> MAASGLDHLKNGYRRRFCRPSRARDINTEQGQNVLEILQDCFEEKSLANDFSTNSTKSVPNSTRKIKDTCIQSPSKECQKSHPKSVPVSSKKKEASLQFVVEPSEATNRSVQAHEVHQKILATDVSSKNTPDSKKISSRNINDHHSEADEEFYLSVGSPSVLLDAKTSVSQNVIPSSAQKRETYTFENSVNMLPSSTEVSVKTKKRLNFDDKVMLKKIEIDNKVSDEEDKTSEGQERKPSGSSQNRIRDSEYEIQRQAKKSFSTLFLETVKRKSESSPIVRHAATAPPHSCPPDDTKLIEDEFIIDESDQSFASRSWITIPRKAGSLKQRTISPAESTALLQGRKSREKHHNILPKTLANDKHSHKPHPVETSQPSDKTVLDTSYALIGETVNNYRSTKYEMYSKNAEKPSRSKRTIKQKQRRKFMAKPAEEQLDVGQSKDENIHTSHITQDEFQRNSDRNMEEHEEMGNDCVSKKQMPPVGSKKSSTRKDKEESKKKRFSSESKNKLVPEEVTSTVTKSRRISRRPSDWWVVKSEESPVYSNS;> MEEQPQMQDADEPADSGGEGRAGGPPQVAGAQAACSEDRMTLLLRLRAQTKQQLLEYKSMVDASEEKTPEQIMQEKQIEAKIEDLENEIEEVKVAFEIKKLALDRMRLSTALKKNLEKISRQSSVLMDNMKHLLELNKLIMKSQQESWDLEEKLLDIRKKRLQLKQASESKLLEIQTEKNKQKIDLDSMENSERIKIIRQNLQMEIKITTVIQHVFQNLILGSKVNWAEDPALKEIVLQLEKNVDMM;> MSPQKRVKNVQAQNRTSQGSSSFQTTLSAWKVKQDPSNSKNISKHGQNNPVGDYEHADDQAEEDALQMAVGYFEKGPIKASQNKDKTLEKHLKTVENVAWKNGLASEEIDILLNIALSGKFGNAVNTRILKCMIPATVISEDSVVKAVSWLCVGKCSGSTKVLFYRWLVAMFDFIDRKEQINLLYGFFFASLQDDALCPYVCHLLYLLTKKENVKPFRVRKLLDLQA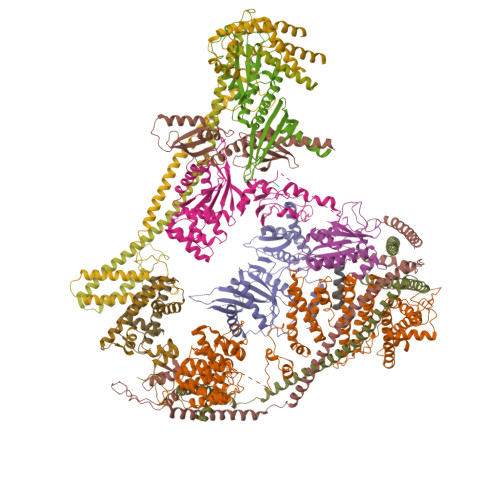KMGMQPHLQALLSLYKFFAPALISVSLPVRKKIYFKNSENLWKTALLAVKQRNRGPSPEPLKLMLGPANVRPLKRKWNSLSVIPVLNSSSYTKECGKKEMSLSDCLNRSGSFPLEQLQSFPQLLQNIHCLELPSQMGSVLNNSLLLHYINCVRDEPVLLRFYYWLSQTLQEECIWYKVNNYEHGKEFTNFLDTIIRAECFLQEGFYSCEAFLYKSLPLWDGLCCRSQFLQLVSWIPFSSFSEVKPLLFDHLAQLFFTSTIYFKCSVLQSLKELLQNWLLWLSMDIHMKPVTNSPLETTLGGSMNSVSKLIHYVGWLSTTAMRLESNNTFLLHFILDFYEKVCDIYINYNLPLVVLFPPGIFYSALLSLDTSILNQLCFIMHRYRKNLTAAKKNELVQKTKSEFNFSSKTYQEFNHYLTSMVGCLWTSKPFGKGIYIDPEILEKTGVAEYKNSLNVVHHPSFLSYAVSFLLQESPEERTVNVSSIRGKKWSWYLDYLFSQGLQGLKLFIRSSVHHSSIPRAEGINCNNQY;> MNQEDLDPDSTTDVGDVTNTEEELIRECEEMWKDMEECQNKLSLIGTETLTDSNAQLSLLIMQVKCLTAELSQWQKKTPETIPLTEDVLITLGKEEFQKLRQDLEMVLSTKESKNEKLKEDLEREQRWLDEQQQIMESLNVLHSELKNKVETFSESRIFNELKTKMLNIKEYKEKLLSTLGEFLEDHFPLPDRSVKKKKKNIQESSVNLITLHEMLEILINRLFDVPHDPYVKISDSFWPPYVELLLRNGIALRHPEDPTRIRLEAFHQ;> MDSYSAPESTPSASSRPEDYFIGATPLQKRLESVRKQSSFILTPPRRKIPQCSQLQEDVDPQKVAFLLHKQWTLYSLTPLYKFSYSNLKEYSRLLNAFIVAEKQKGLAVEVGEDFNIKVIFSTLLGMKGTQRDPEAFLVQIVSKSQLPSENREGKVLWTGWFCCVFGDSLLETVSEDFTCLPLFLANGAESNTAIIGTWFQKTFDCYFSPLAINAFNLSWMAAMWTACKMDHYVATTEFLWSVPCSPQSLDISFAIHPEDAKALWDSVHKTPGEVTQEEVDLFMDCLYSHFHRHFKIHLSATRLVRVSTSVASAHTDGKIKILCHKYLIGVLAYLTELAIFQIE;> MSVLRPLDKLPGLNTATILLVGTEDALLQQLADSMLKEDCASELKVHLAKSLPLPSSVNRPRIDLIVFVVNLHSKYSLQNTEESLRHVDASFFLGKVCFLATGAGRESHCSIHRHTVVKLAHTYQSPLLYCDLEVEGFRATMAQRLVRVLQICAGHVPGVSALNLLSLLRSSEGPSLEDL;> MDETVAEFIKRTILKIPMNELTTILKAWDFLSENQLQTVNFRQRKESVVQHLIHLCEEKRASISDAALLDIIYMQFHQHQKVWEVFQMSKGPGEDVDLFDMKQFKNSFKKILQRALKNVTVSFRETEENAVWIRIAWGTQYTKPNQYKPTYVVYYSQTPYAFTSSSMLRRNTPLLGQALTIASKHHQIVKMDLRSRYLDSLKAIVFKQYNQTFETHNSTTPLQERSLGLDINMDSRIIHENIVEKERVQRITQETFGDYPQPQLEFAQYKLETKFKSGLNGSILAEREEPLRCLIKFSSPHLLEALKSLAPAGIADAPLSPLLTCIPNKRMNYFKIRDK;> MEQANPLRPDGESKGGVLAHLERLETQVSRSRKQSEELQSVQAQEGALGTKIHKLRRLRDELRAVVRHRRASVKACIANVEPNQTVEINEQEALEEKLENVKAILQAYHFTGLSGKLTSRGVCVCISTAFEGNLLDSYFVDLVIQKPLRIHHHSVPVFIPLEEIAAKYLQTNIQHFLFSLCEYLNAYSGRKYQADRLQSDFAALLTGPLQRNPLCNLLSFTYKLDPGGQSFPFCARLLYKDLTATLPTDVTVTCQGVEVLSTSWEEQRASHETLFCTKPLHQVFASFTRKGEKLDMSLVS;> MDAELAEVRALQAEIAALRRACEDPPAPWEEKSRVQKSFQAIHQFNLEGWKSSKDLKNQLGHLESELSFLSTLTGINIRNHSKQTEDLTSTEMTEKSIRKVLQRHRLSGNCHMVTFQLEFQILEIQNKERLSSAVTDLNIIMEPTECSELSEFVSRAEERKDLFMFFRSLHFFVEWFEYRKRTFKHLKEKYPDAVYLSEGPSSCSMGIRSASRPGFELVIVWRIQIDEDGKVFPKLDLLTKVPQRALELDKNRAIETAPLSFRTLVGLLGIEAALESLIKSLCAEENN;> MSGKANASKKNAQQLKRNPKRKKDNEEVVLSENKVRNTVKKNKNHLKDLSSEGQTKHTNLKHGKTAASKRKTWQPLSKSTRDHLQTMMESVIMTILSNSIKEKEEIQYHLNFLKKRLLQQCETLKVPPKKMEDLTNVSSLLNMERARDKANEEGLALLQEEIDKMVETTELMTGNIQSLKNKIQILASEVEEEEERVKQMHQINSSGVLSLPELSQKTLKAPTLQKEILALIPNQNALLKDLDILHNSSQMKSMSTFIEEAYKKLDAS;> MPVKRSLKLDGLLEENSFDPSKITRKKSVITYSPTTGTCQMSLFASPTSSEEQKHRNGLSNEKRKKLNHPSLTESKESTTKDNDEFMMLLSKVEKLSEEIMEIMQNLSSIQALEGSRELENLIGISCASHFLKREMQKTKELMTKVNKQKLFEKSTGLPHKASRHLDSYEFLKAILN;> MADHNPDSDSTPRTLLRRVLDTADPRTPRRPRSARAGARRALLETASPRKLSGQTRTIARGRSHGARSVGRSAHIQASGHLEEQTPRTLLKNILLTAPESSILMPESVVKPVPAPQAVQPSRQESSCGSLELQLPELEPPTTLAPGLLAPGRRKQRLRLSVFQQGVDQGLSLSQEPQGNADASSLTRSLNLTFATPLQPQSVQRPGLARRPPARRAVDVGAFLRDLRDTSLAPPNIVLEDTQPFSQPMVGSPNVYHSLPCTPHTGAEDAEQAAGRKTQSSGPGLQKNSPGKPAQFLAGEAEEVNAFALGFLSTSSGVSGEDEVEPLHDGVEEAEKKMEEEGVSVSEMEATGAQGPSRVEEAEGHTEVTEAEGSQGTAEADGPGASSGDEDASGRAASPESASSTPESLQARRHHQFLEPAPAPGAAVLSSEPAEPLLVRHPPRPRTTGPRPRQDPHKAGLSHYVKLFSFYAKMPMERKALEMVEKCLDKYFQHLCDDLEVFAAHAGRKTVKPEDLELLMRRQGLVTDQVSLHVLVERHLPLEYRQLLIPCAYSGNSVFPAQ;> MAPRGRRRPRPHRSEGARRSKNTLERTHSMKDKAGQKCKPIDVFDFPDNSDVSSIGRLGENEKDEETYETFDPPLHSTAIYADEEEFSKHCGLSLSSTPPGKEAKRSSDTSGNEASEIESVKISAKKPGRKLRPISDDSESIEESDTRRKVKSAEKISTQRHEVIRTTASSELSEKPAESVTSKKTGPLSAQPSVEKENLAIESQSKTQKKGKISHDKRKKSRSKAIGSDTSDIVHIWCPEGMKTSDIKELNIVLPEFEKTHLEHQQRIESKVCKAAIATFYVNVKEQFIKMLKESQMLTNLKRKNAKMISDIEKKRQRMIEVQDELLRLEPQLKQLQTKYDELKERKSSLRNAAYFLSNLKQLYQDYSDVQAQEPNVKETYDSSSLPALLFKARTLLGAESHLRNINHQLEKLLDQG;> MALSTIVSQRKQIKRKAPRGFLKRVFKRKKPQLRLEKSGDLLVHLNCLLFVHRLAEESRTNACASKCRVINKEHVLAAAKVILKKSRG> KVFERCELARTLKRLGMDGYRGISLANWMCLAKWESGYNTRATN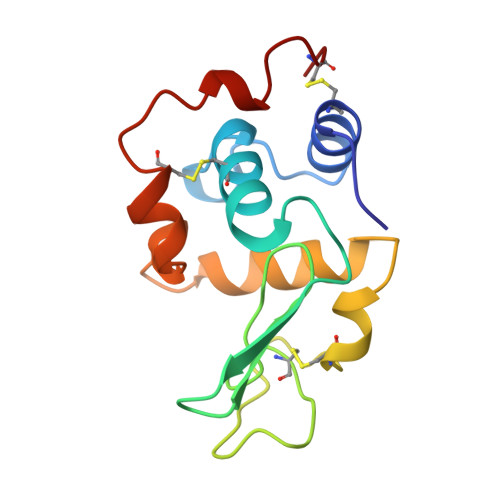YNAGDRSTDYGIFQINSRYWCNDGKTPGAVNAAHLSCSALLQDNIADAVAAAKRVVRDPQGIRAWVAWRNRCQNRDARQYVQGCGV> QNGYENPTYK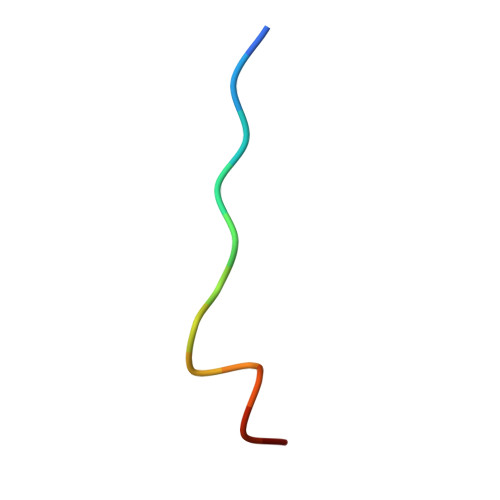FFE> GSHMVPAALPQLTPTLVSLLEVIEPEVLYAGYDSSVPDSAWRIMTTLNMLGGRQVIAAVKWAKAIPGFRNLHLDDQMTLLQYSWMSLMAFALGW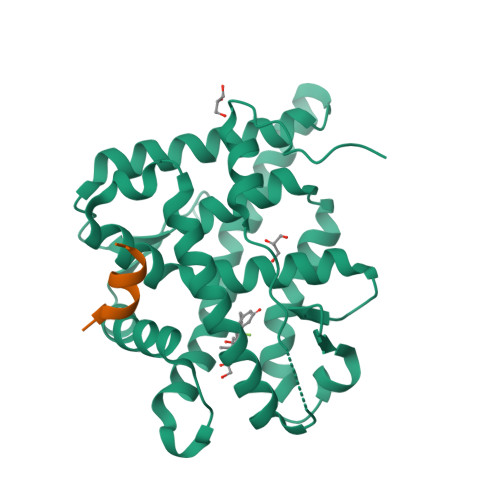RSYRQASGNLLCFAPDLIINEQRMTLPCMYDQCKHMLFISTELQRLQVSYEEYLCMKTLLLLSSVPKEGLKSQELFDEIRMTYIKELGKAIVKREGNSSQNWQRFYQLTKLLDSMHDVVENLLSYCFQTFLDKSMSIEFPEMLAEIITNQIPKYSNGNIKKLLFHQK;> KENALLRYLLDKD> GAENESTPIQQLLEHFLRQLQRKDPHGFFAFPVTDAIAPGYSMIIKHPMDF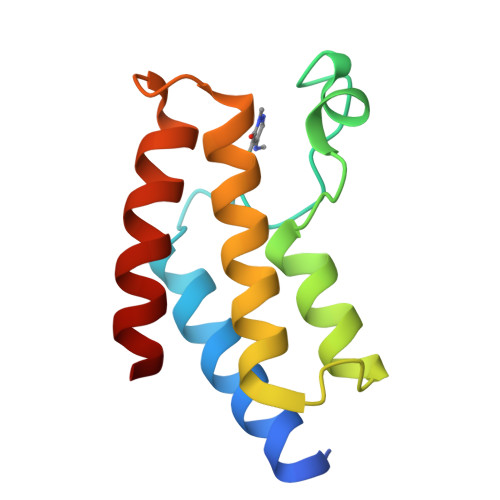GTMKDKIVANEYKSVTEFKADFKLMCDNAMTYNRPDTVYYKLAKKILHAGFKMMS> QSTQIKIERDNYGVPHIYANDTYSLFYGYGYAVAQDRLFQMEMAKRSTQGTVSEVFGKDYISFDKEIRNNYWPDSIHKQINQLPSQEQDILRGYADGMNAWIKQINTKPDDLMPKQFIDYDFLPSQWTSFDVAMIMVGTLANRFSDM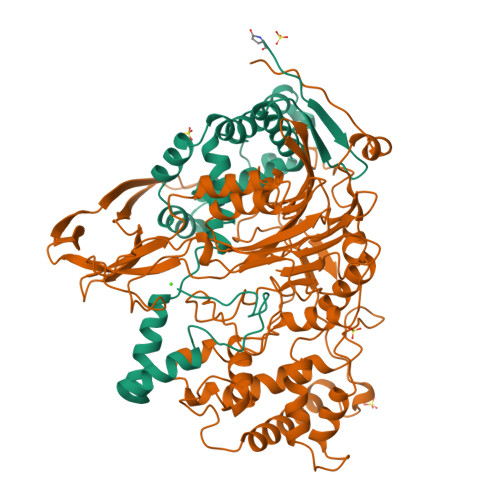NSEIDNLALLTALKDKYGEQLGVEFFNQINWLNNPNAPTTISSEEFTYSDSQKTKNIS;> SNVWLVGKTKASGAKAILLNGPQFGWFNPAYTYGIGLHGAGFNIVGNTPFAYPAILFGHNGHVSWGSTAGFGDGVDIFAEQVSPEDPNSYLHQGQWKKMLSRQETLNVKGEQPITFEIYRTVHGNVVKRDKTTHTAYSKARAWDGKELTSLMAWVKQGQAQNWQQWLDQAQNQALTINWYYADKDGNIGYVHTGHYPDRQINHDPRLPVSGTGEWDWKGIQPFANNPKVYNPKSGYIANWNNSPAKNYPASDLFAFLWGSADRVKEIDNRIEAYDKLTADDMWAILQQTSRVDLNHRLFTPFLTQATQGLPSNDNSVKLVSMLQQWDGINQLSSDGKHYIHPGSAILDIWLKEMLKATLGQTVPAPFDKWYLASGYETTQEGPTGSLNISTGAKLLYESLLEDKSPISQSIDLFSGQPQNDVIRKTLNTTYQKMIEKYGDNPANWQTPATALTFRENNFFGIPQALPQENFHQNEYHNRGTENDLIVFTEEGVSAWDVVAPGQSGFISPQGKPSPHYQDQLSLYQQFGKKPLWLNSEDVAPYIESTETLIIER>[4x]GSFDLEDVQPNKTTGVSKEEYKDVETDKKVKEQLGELMEPALGYVVKVPVSQSGVKRTEISNPEAITDEDLNKIPNYEIIKGVAYPNYGELVDKTAAETMKYVRSGYVIDVYHSGTRDKGYVFYKGITPSKELPQGPALTYQGEWDFTSDANLNNEEGRPTYLNDDYYTTAIGKRAGLVSGDAKPSKHKYTSQFKVDFATKKMTGKLSDKEKTIYTVNADIRGNRFTGSATASDKDKGKGASYNFFSVDSQSLEGGFYGPKAEEMAGKFVADDKSLFAVFSAKHNASNVNTVRIIDASKIDLTNFSISELTNFGDASVLIIDGKKMELAGSEFTNKHTIDINGKKMVAVACCSNLEYMKFGQLWQQTEGEKQVKDNSLFLQGERTATDKMPKDGNYKYIGTWDAQVSKENNYWVATADDDRKAGYRTEFDVDFGSKNLSGKLFDKNGVNPVFTVNAKIDGNGFTGEAKTSDAGFVLDPGSLRH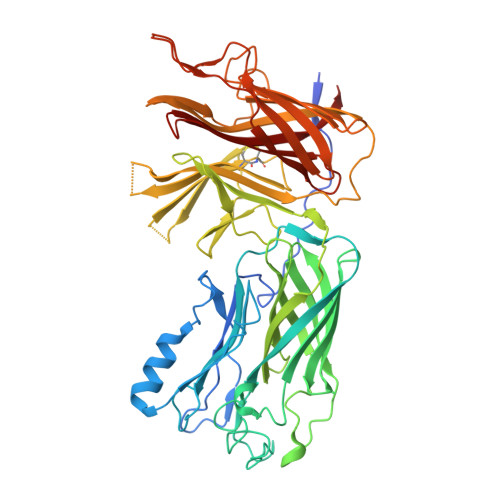DNVKFSDVAVSGGFYGPTAAELGGQFRYQSDNGSVGVGAVFGAKQQVKK>SHEQFRAALQLVVDPGDPRSYLDNFIKIGEGSTGIVCIATVRSSGKLVAVKKMDLRKQQRRELLFNEVVIMRDYQHENVVEMYNSYLVGDELWVVMEFLEGGALTDIVTHTRMNEEQIAAVCLAVLQALSVLHAQGVIHRDIKSDSILLTHDGRVKLSDFGFCAQVSKEVPRRKSLVGTPYWMAPELISRLPYGPEVDIWSLGIMVIEMVDGEPPYFNEPPLKAMKMIRDNLPPRLKNLHKVSPSLKGFLDRLLVRDPAQRATAAELLKHPFLAKAGPPASIVPLMRQNRTR[2x]

PAKs are serine/threonine protein kinases that are regulated by Rho GTPases of the Cdc42 and Rac families (Knaus et al., 1995; Manser et al., 1994; Martin et al., 1995). In humans, the PAK family comprises six members, which are classified into groups I (PAK1, -2, and -3) and II (PAK4, -5, and -6) based on their domain architecture and regulatory properties (Bokoch, 2003; Jaffer and Chernoff, 2002; Kumar et al., 2006; Zhao and Manser, 2005). Group II PAKs (PAK4–6) regulate a wide variety of cellular functions, and PAK deregulation has been linked to tumor development. Comparison of five high-resolution crystal structures comprising the kinase domains of all three monophosphorylated, enzymatically active group II PAK family members revealed a number of catalytically productive and nonproductive conformers presumably representing snapshots of catalytic domain movements during catalysis.

Finally, we solved the structure of noncatalytically productive apo structures of PAK4, PAK5, and PAK6. In the apo structure of PAK4, large regions of the kinase domain were disordered, including parts of helix αC, the glycine-rich loop, as well as part of the activation segment. Evidently, the activation segments remain quite flexible in that crystal form despite the presence of the activating phosphorylation site at residue Ser474. The significant disorder of PAK4 in this crystal form precluded detailed structural comparisons with other PAK family members.Here we report seven high-resolution cryo-EM structures of filamentous peptide nanotubes based on a cross-α supramolecular architecture that provide insight into the designability of helical peptide filaments. A structural interaction is identified based on an appropriately placed pair of arginine residues (RxxxR) within the corresponding peptide sequences. This local interaction motif, designated as an arginine clasp, is robust within the context of these cross-α assemblies and can guide the coalescence of helical protofilaments into structurally defined cross-α nanotubes. In contrast to most structurally characterized filaments based on synthetic α-helical coiled-coils, the chain axes of the helical protomers are oriented in a plane nearly perpendicular to the long axis of the assembly.

Arginines were placed in an i,i + 3 (RxxR) arrangement within a heptad repeat located proximal to the N-terminus. The sequence at the axial interface was conserved in order to maintain the cross-α stacking interactions within a protofilament. The resultant peptide was designated as 29-20-2 using the same (x-y-z) nomenclature described above, with the value of z equal to 2 for the RxxR motif. The 29-20-2 peptide adopted an α-helical conformation in solution and. formed high aspect-ratio tubular filaments. However, the observed widths of the filaments were significantly larger, circa 12 nm, than the corresponding values for peptides in the (x-y-3) series. A 3.8-Å resolution helical reconstruction from the corresponding cryo-EM images afforded an atomic model for the 29-20-2 filament. Unexpectedly, the filament formed a double-walled cross-α nanotube that was similar in structure to that of the Form II filament and a structurally related mutant. Remarkably, the arginine residues in RxxR motif were not involved in the lateral interactions between cross-α helical protofilaments. Instead, cohesive interactions were mediated through hydrogen-bonding between the N- and C-terminal glutamine residues from helices on laterally adjacent protofilaments, as in the Form II-related structures. The structural analysis of the 29-20-2 filament provided evidence that the formation of the arginine clasp interaction required not only the presence of the two arginines, but also the correct orientation, RxxxR, of the corresponding residues within the sequences of the respective helical protomers. The relatively minor substitution of an RxxR motif for an RxxxR motifs drove the lateral association down an alternative pathway that resulted in formation of a double-walled nanotube in which lateral interactions occurred between terminal glutamine residues.

>[150x]QAEILEADARILRAYAEILKAHAEILKAQ>HHHHHHENLYFQGMAVSPSPLRIFTAGGTIDEDYRLEENGLVVGDPFVAEVLKTARLAGAVSIVALSRKDSLDFTEADREAIGRAVGQAVEDHILLTHGTDTMVETARYLGGLPELAGKTVVLSGAMVPGRVGGSDAAFNIGFACAAALMLAPGVYIAMHGKVFDPAKTRKNRGLGRFEPIDDQE[2x]

L‐Asparaginases (ASNases) catalyze the hydrolysis of L‐Asn to L‐Asp and ammonia. In contrast, the chain of ASNase from Rhodospirillum rubrum, reported here and referred to as RrA, consists of only 172 amino acid residues. RrA is homologous to the N‐terminal domain of typical bacterial class 1 ASNases and exhibits millimolar affinity for L‐Asn. Crystal structures of the wild‐type RrA, both with and without bound L‐Asp, as well as structures of several RrA mutants, reveal topologically unique tetramers.

A distinctive feature of RrA is the presence of Lys19 within the lining of the substrate‐binding site. We probed the importance of this residue by mutating it to L‐Ala, L‐Glu, and L‐Gln. Crystals of RrA(K19E) were isomorphous with those of RrA(K19Q) and were obtained only in the absence of L‐Asp. The kinetic data, even when reduced to approximate turnover numbers, demonstrate that Lys19 plays an important role during catalysis and its mutation reduces the rate of catalysis by two or more orders of magnitude. Further studies are necessary to explain the differences between the activities of the K19A, K19E, and K19Q variants.>MGFKSWITEKLNPGQRIIRDMEPVSHRTNRKPFTTGQAYSKIEILNRTANMVIDSAAECSYTVGDKYNIVTYANGVKTKTLDTLLNVRPNPFMDISTFRRLVVTDLLFEGCAYIYWDGTSLYHVPAALMQVEADANKFIKKFIFNNQINYRVDEIIFIKDNSYVCGTNSQISGQSRVATVIDSLEKRSKMLNFKEKFLDNGTVIGLILETDEILNKKLRERKQEELQLDYNPSTGQSSVLILDGGMKAKPYSQISSFKDLDFKEDIAGFNKSICLAFGVPQVLIDGGNNANIRPNIELFYYMTIIPMLNKLTSSLTFFFGYKITPNTKEVAALTPDKEAEAKHLTSLVNNGIMTGNEARLELNLEPLDDEQMNRIRIPANVAGSATGVSGQEGGRPQGSTEGDKE[4x];>[4x]MQIITAEDYRLYGGLKRPELESGVEMMITAANALITSLLGMDDADAVDQLINTKPTRKKYFLSSPSATSVTKMTINDKEIDPEQYKLYSDGVILLKFSPPEGYMDVEYTQGGFNPIPEDLKLAACMLVDHWHKQDYRQAKTIGGETVTFNNTKSGIPEHIRTIIEVYRRV;>[2x]MDHRTSIAQALVDRIAQQMDGSQPDEYFNNLYGNVSRQTYKFEEIREFPYVAVHIGTETGQYLPSGQQWMFLELPILVYDKEKTDIQEQLEKLVADIKTVIDTGGNLEYTVSKPNGSTFPCEATDMSITSVSTDEGLLAPYGLAEINVTVRYQPPRRSLRR;> MTDKLIRELLIDVKQKGATRTAKSIENVSDALENAAAASELTNEQLGKMPKTLYSIERAADRAAKSLTKMQASRGMAGITKSIDSIGAKLDDLSIAMIEVADKLEAGFDGVSRSVKVMGNDVAAATEKVQDRLYDTNRVLGGTARGFNDTAGAAGRASRAIGNTSGSARGATRDFAAMAKVGGGLPLLYAAIASNIFVLQSAFEQLKLGDQLNRLEEFGVIVGTQTGTPVQSLARSLQEAAGYAISFEEAMRQASSASAYGFDAEQLNKFGLVARRAAAVLGVDMTDALNRVIKGVSKQEIELLDELGVTIRLNDAYADYVKQLNAANTGITYNINSLTTFQKQQAYANAVIAESTKRFGYLDEVLRATPWEQFAANADAALRTIQQAAAKYLGPVIDAINTVFYTSQASISAEAARAQEQTNKQIDPTNVGAVALSLSASEEGYNKALDMYKESLDKRNKLKSEFDKRMEQADFYTKLAIRQVGEGIPAGLATAGASEANKKFVEETAAMGLQVARLDKEVTDSTENLNAWKSAYQAAGAAAAKANPEFQKQINLQRDTTDPGAVYDFNSTVLKGLTEQQKAYNQTKKTASDLANDIQNVAQNTDTAAKTSATLADAIKNIESLSLGTGKSADEYVKNLNLGYNTLSEMKTASQALSEYVKLTGNETKNQLAVQQKIADVYNQTKDKEKAQEAGRRLELQQLEEQEAALRRVLQTNQGNKAVEREIEKIQLEKIKLTNQGMEAQKKVKDYTDKILGVDREIALLNNRTMTDTQYRLAQLNLELTIEKEKYEWYTKQADKQKEAEQSRRAQAQIEREIWKFHQDQQAEMTSKRQEAFENTLTSMFPLAGEMQKMEMQLDFYTQMKELTKDNANEQMRWNAEIAKTRAQMSALTAQRNAQMQSSVGSSLGAVYTPTTGLSGEDKKFADMGNQLASYDQAISKLSELNSEATAVAQSMGNLANAMIQFSQGSLDTTSTIAVGMQTVASMIQYSTSQQVSAIDQAIAAEQKRDGKSEASKAKLKKLEAEKLKIQQDAAKKQIIIQTAVAVMQAATAVPYPFSIPLMIAAGLAGALALAQASSASGMSSIGDSGADTASYLTLGERQKNIDVSMSANAGELSYVRGDKGIGNANSFVPRAEGGNMYPGVSYQMGEHGTEVVTPMVPMKATPNDELKNSSNSTAGRPIILNISAMDAASFREFASSNSGALRDAVELALNENGASLKTLGNS

The T5 family of viruses are tailed bacteriophages characterized by a long non-contractile tail. The bacteriophage DT57C is closely related to the paradigmal T5 phage, though it recognizes a different receptor (BtuB) and features highly divergent lateral tail fibers (LTF). We present a composite map determined by electron cryo-microscopy (cryo-EM) at resolutions ranging between 2.9 Å to 4.9 Å of the entire T5-like phage particle DT57C, and atomic models comprising its core structural proteins. Our results provide a complete atomic structure of a T5-like phage, provide insights into the process of DNA ejection as well as a structural basis for the design of engineered phages and future mechanistic studies.

The reconstruction of the capsid-tail interface, here referred to as the neck region, reached a resolution of 3.4 Å and revealed the presence of three proteins that enable the transition from capsid to the tail tube. The portal protein (PrtP) forms a dodecameric ring, which replaces one of the MCP pentamers of the capsid. The PrtP ring interacts directly with a ring of head completion protein (HCP), also dodecameric. The interface is completed by a hexameric ring of tail completion protein (TCP), which connects to the first trimeric ring of tail tube protein (TTP). At the HCP-TCP interface level, there is a steep reduction in the diameter of the density attributed to the DNA, suggesting that DNA is locked in the PrtP-HCP lumen through interactions with the DI of the HCP ring even before attachment of the tail to packed viral heads. Since the negatively charged DNA should experience significant repulsive force when passing through this region of the portal complex, the dynamic nature of the HCP DI β-hairpins may contribute towards preventing premature DNA release. Furthermore, our cryo-EM map resolved the secondary structure of the N-terminal part of the TMP as a trimeric α-helical coiled-coil. Second, we found that the neck tunnel at the HCP-TCP interface is open in the pre-ejection DNA state and remains open after DNA release.> TLTVQARQLLSGIVQQQNDLLRAIEAQQHLLQLTVWGIKQLQARSGGRGGWME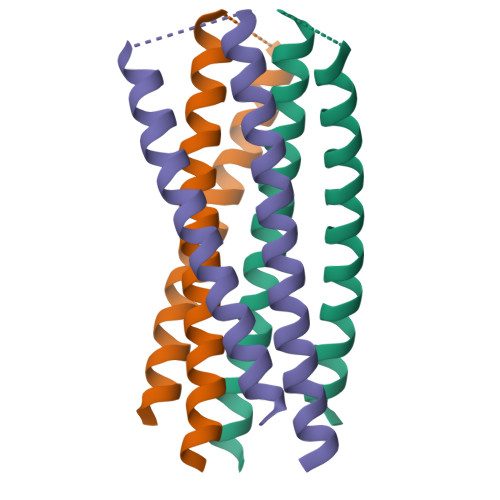WDREINNYTSLIHSLIEESQNQQEKNEQELLEL>MHKITLIPGDGIGPSIVDAAVKVIEATGVQVQWDTQSAGMAAVEKFGTPLPDATLDSIRANRICFKGPLTTPVGGGYRSVNVTLRQALNLYANVRPAISFEGTDTAFSDVNLVTVRENTEGLYAGIEHFIKVD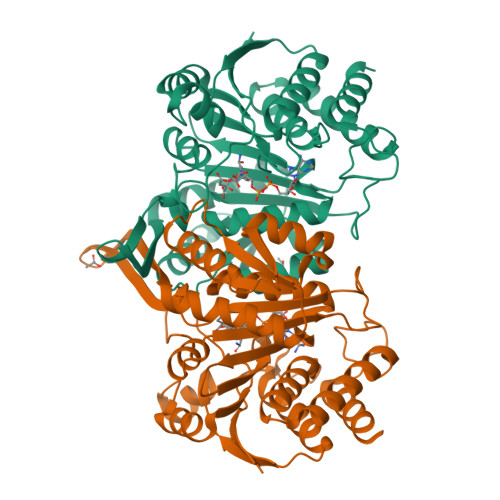EEKIAAESIAVVTRKGSERIIRYAFDYARRARRKKVTLVHKANILKCTSGLFLEIGREIAKEYPDIEFDDRIVDACSMQMVMQPQRFDVLVTTNLFGDILSDLAAGLIGGLGLTAGANIGTDAALFEAVHGSAPDIADKGIANPTAMIMAGAMMLEHIGEPDAARRIERAVREVIEDGRSVTPDLAKDSPCGTAQMAEAIVERVRQA[2x]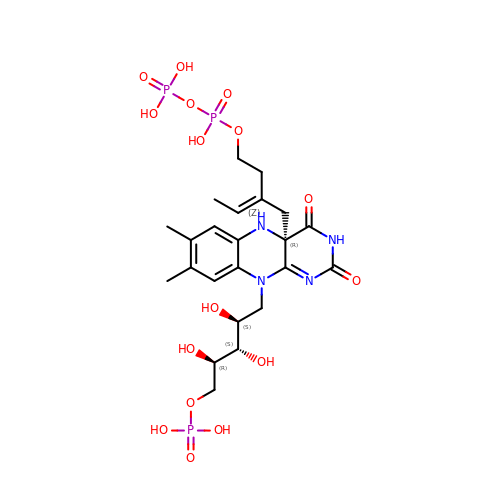1-deoxy-1-[(4aR)-4a-[(2Z)-2-(2-{[(S)-hydroxy(phosphonooxy)phosphoryl]oxy}ethyl)but-2-en-1-yl]-7,8-dimethyl-2,4-dioxo-3,4,4a,5-tetrahydrobenzo[g]pteridin-10(2H)-yl]-5-O-phosphono-D-ribitol | C23 H35 N4 O16 P3 | OAOWJIIZSRFUAL-QCJQWHCGSA-N> SPVVVVTGASRGIGKAIALSLGKAGCKVLVNYARSAKAAEEVSKQIEAYGGQAITFGGDVSKEADVEAMMKTAIDAWGTIDVVVNNAGITRDTLLIRMKKSQWDEVIDLNLTGVFLCTQAATKIMMKKRKGRIINIASVVGLIGNIGQANYAAAKAGVIGFSKTAAREGASRNINVNVVCPGFIASDMTAKLGEDMEKKIL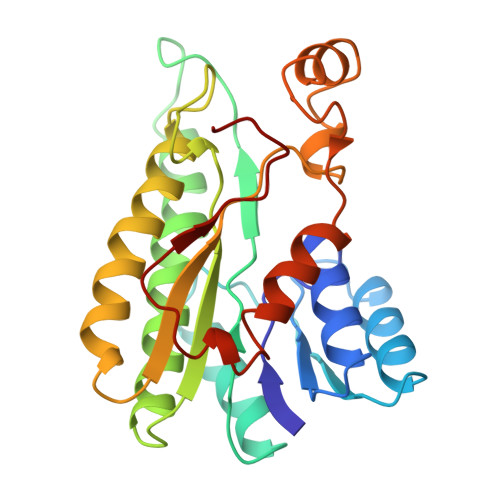GTIPLGRTGQPENVAGLVEFLALSPAASYITGQAFTIDGGIAI> MQSSTSTDQHVLHHMDPHRFTSQIPTATSSQLRRRNSTNQGLTDMINKSIARNTISGTGIPTGGINKNKRTRSTVAGGTNGTALALNDKSNSRNSVSRLSINQLGSLQQHLSNRDPRPLRDKNFQSAIQEEIYDYLKKNKFDIETNHPISIKFLKQPTQKGFIIIFKWLYLRLDPGYGFTKSIENEIYQILKNLRYPFLESINKSQISAVGGSNWHKFLGMLHWMVRTNIKLDMCLNKVDRSLINQNTQEITILSQPLKTLDEQDQRQERYELMVEKLLIDYFTESYKSFLKLEDNYEPSMQELKLGFEKFVHIINTDIANLQTQNDNLYEKYQEVMKISQKIKTTREKWKALKSDSNKYENYVNAMKQKSQEWPGKLEKMKSECELKEEEIKALQSNISELHKILRKKGISTEQFELQNQEREKLTRELDKINIQSDKLTSSIKSRKLEAEGIFKSLLDTLRQYDSSIQNLTRSRSQLGHNVNDSSLKINISENLLDRDFHEGISYEQLFPKGSGINESIKKSILKLNDEIQERIKTIEKDNITLEKDIKNLKHDINEKTQINEKLELELSEANSKFELSKQENERLLVAQRIEIEKMEKKINDSNLLMKTKISDAEELVTSTELKLEELKVDLNRKRYKLHQQVIHVIDITSKFKINIQSSLENSENELGNVIEELRNLEFETEHNVTN;> MSRNQDVFPILDLQELVICLQSCDFALATQENISRPTSDYMVTLYKQIIENFMGISVESLLNSSNQETGDGHLQEENENIYLDTLNVLVLNKICFKFFENIGVQDFNMTDLYKPEAQRTQRLLSAVVNYARFREERMFDCNSFILQMESLLGQLRSKFDDYNLIQQQLKQYEDVDGDNIPDEQELQKLEEQNKELEIQLKKLTKIQETLSIDYNDYKISKQSIFKDLEALSFQIVELESNRDKLIKISNTDMEELSEGIKELNDLLIQRKKTLDDLTAQQKNLQDTVTTFETIISELYDVLRIISSEVQESNRTETELVGLKQNLINNKLKLMNVLETGIMYKLEILQEQLDLQLKNLEKLSQDTKEESRLNDTKLMDLQIKYENEIKPKIDKTDIFIQEELISGKINKLNDEIKQLQKDFEVEVKEIEIEYSLLSGHINKYMNEMLEYMQ;> MSEDKAKLGTTRSATEYRLSIGSAPTSRRSSMGESSSLMKFADQEGLTSSVGEYNENTIQQLLLPKIRELSDSIITLDSNFTRLNFIHESLADLNESLGSLLYGIMSNSWCVEFSQAPHDIQDDLIAIKQLKSLEDEKNNLVMELSNMERGIKRKKDEQGENDLAKASQNKQFNQPLFPSSQVRKYRSYDNRDKRKPSKIGNNLQVENEEDYEDDTSSEASFVLNPTNIGMSKSSQGHVTKTTRLNNNTNSKLRRKSILHTIRNSIASGADLPIENDNVVNLGDLHPNNRISLGSGAARVVNGPVTKNRNSMFSGRAERKPTESRHSVAKKTEKKINTRPPFR;> MSEQSQLDDSTIDKLIPQIFNEMRSNLNNTTNKFPKSTGGGASDNISANSNSIRSFNSITTQSLLKESESLDKITAMIKNVTAALKNNLPVYVNQVHEVCKSTNSILDSWINIHSQAGYIHKLMSDQTYLKLINDRLHNENVNTNDEDGSTLHNVIALKKKEILDLRQKLENRKGEKDAAPAKPPNQGLNPRYGVQSGRRPVPSAGISNNGRVRKTHVPASKRPSGIPRVTNRWTKPTASSSRKMFR;> MDSIDEQIAIKRKELQSLQKITSLTDGLKIQLTELNEQIKEMGMNADSVAQLMNNWDSIINNISQASLGLLQYAEGDYEIGPWKDSKKKESEQSNETGLEAQENDKNDEDNDEDEDLVPLPETMVRIRVDGNE;> MMASTSNDEEKLISTTDKYFIEQRNIVLQEINETMNSILNGLNGLNISLESSIAVGREFQSVSDLWKTLYDGLESLSDEAPIDEQPTLSQSKTK;> MENPHEQVQANILSRIIGNVKRLNESVAILNQELVTINNRNKNLEIMGAICDNYHSSVQFNLEATNNKKPPL;> MEHNLSPLQQEVLDKYKQLSLDLKALDETIKELNYSQHRQQHSQQETVSPDEILQEMRDIEVKIGLVGTLLKGSVYSLILQRKQEQESLGSNSK;> MGESLDRCIDDINRAVDSMSTLYFKPPGIFHNAILQGASNK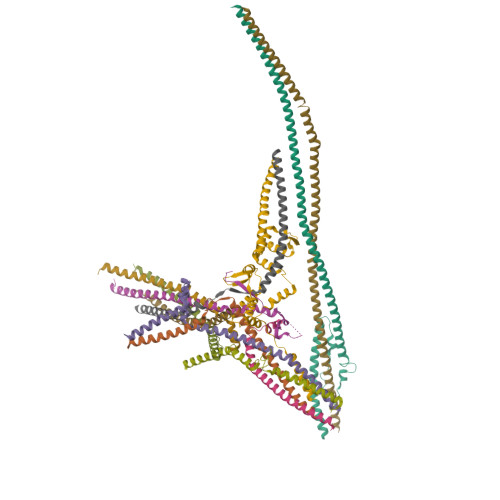ASIRKDITRLIKDCNHDEAYLLFKVNPEKQSVSRRDGKEGVFDYVIKRDTDMKRNRRLGRPGEKPIIHVPKEVYLNKDRLDLNNKRRRTATTSGGGLNGFIFDTDLIGSSVISNSSSGTFKALSAVFKDDPQIQRLLYALENGSVLMEEESNNQRRKTIFVEDFPTDLILKVMAEVTDLWPLTEFKQDYDQLYHNYEQLSSKLRFIKKEVLLQDDRLKTMSQYHPSSSHDVAKIIRKEKDEIRRLEMEIANLQE;> MDSASKEETLEKLDQEITVNLQKIDSNLSFCFHKITQDIIPHVATYSEICERIMDSTEWLGTMFQETGLVNLQANAAAPVGNAPVKSLVSNNVGIFPTSAEEASRQSQTDNGPNEADSAVHVNRDVHSMFNNDSIDDFHTANITSTGQILKLPDSSDEDTGSEAVPSREQTDLTGEGHGGADDEQDESTIQRQSRKRKISLLLQQQYGSSSSMVPSPIVPNKMRKQLAHEEHINNDGDNDDENSNNIESSPLKQGHHHPKGQADDNNEGPDEEESTKEVPKPGTIIHFSTNR;> MNANKQRQYNQLAHELRELQTNLQETTKQLDIMSKQCNENLVGQLGKVHGSWLIGSYIYYMEQMLGKTQ;> MTDALEQSVLALEGTVSVLKDSVESLKCANEPSTNLASTMLQTKRVFRLVPEYDVERSKLDLIEEVEPLVRTLGDKLRKSMGRMQRELDTLQQTYELNDLRLKKNISMDDDDALNSPDMGQEYEGRDADDVVMMASSTNEELEELKKLKEKKKQLENKLEILKQK> MVNFNLKANTTYLRLVEENDAEFICTLRNNDKLNTYISKSTGDIKSQAEWIRNYKNRENNGEEYYFIIFRSDDQSPIGTVRLYDFHENPKSFCWGSWILNEHKTKYAAVESALLVYEAGFSTLGFEQSHFEVMKGNDKVHSFHLKMGAQKISEDDENIYYIFPKSKYKENK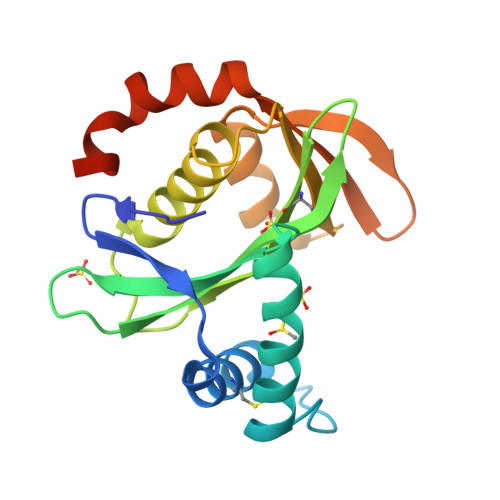IQYARFLGKLEHHHHHH> GEIEFIESSKDAGFPVINTPSKTKLEPSVFHQVFEGNKEPAVLRSGDPRLKANFEEAIFSKYIGNVNTHVDEYMLEAVDHYAGQLATLDISTEPMKLEDAVYGTEGLEALDLTTSAGYPYVALGIKKRDILSKKTKDLTKLKECMDKYGLNLPMVTYVKDELRSIEKVAKGKSRLIEASSLNDSVAMRQTFGNLYKTFHLNPGVVTGSAVGCDPDLFWSKIPVMLDGHLIAFDYSGYDASLSPVWFACLKMILEKLGYTHKETNYIDYLCNSHHLYRDKHYFVRGGMPSGCSGTSIFNSMINNIIIRTLMLKVYKGIDLD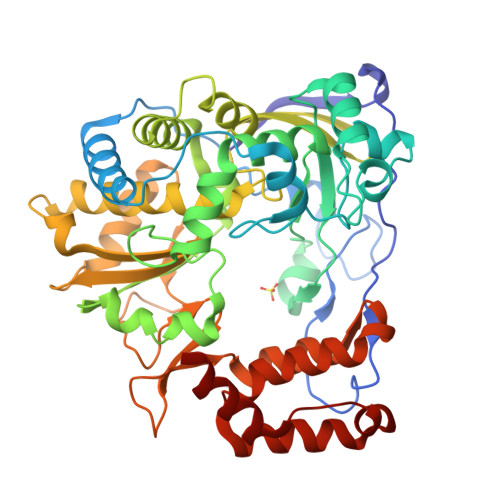QFRMIAYGDDVIASYPWPIDASLLAEAGKGYGLIMTPADKGECYNEVTWTNVTFLKRYFRADEQYPFLVHPVMPMKDIHESIRWTKDPKNTQDHVRSLCLLAWHNGEHEYEEFIRKIRSVPVGRCLTLPAFSTLRRKWLDSF Here, we present the first report on the identification and characterization of a lectin from S. apiospermum named SapL1. SapL1 was found using bioinformatics as a homolog to the conidial surface lectin FleA from Aspergillus fumigatus known to play a role in the adhesion to host glycoconjugates present in human lung epithelium. As expected from its homology with FleA, SapL1 recognizes fucosylated oligosaccharides independently of the fucose linkage. We finally demonstrated that SapL1 binds to bronchial epithelial cells in a fucose-dependent manner.

SapL1 was co-crystallized with α-methyl-fucoside and the structure of the complex was solved by molecular replacement at 2.3 Å resolution in the P21 space group using the coordinates of FleA (PDB code 4D4U34) as the search model. The asymmetric unit contained two monomers, assembled as a dimer with all 295 amino acids visible apart of the N-terminal methionine. SapL1 folds into the canonical six-bladed β-propeller with six-binding sites at the interface between blades typical for this family of lectin. Due to divergence in the tandem repeat sequence forming each blade of the propeller, the six binding sites of SapL1 monomer are not equivalent, but they share important conserved features. Hydrophobic interactions are observed between the C6 of the fucose and at least three residues of the protein (mainly isoleucine, tryptophan/tyrosine and leucine). The O2 and O3 hydroxyls make strong hydrogen bonds with a conserved triad of amino acids consisting of an arginine, a glutamic acid and a tryptophan. The O2 hydroxyl seemed to be the most versatile position, since it established interactions with an adjacent loop only present in four of the six binding sites (BPs 2, 4, 5 and 6). This is particularly interesting since the binding pockets that do not contain this loop (BPs 1 and 3) were mostly occupied by glycerol instead of fucose, indicating that those interactions could be responsible for enhancing the affinity and should be explored for development of inhibitors. The overall fold of SapL1 and FleA as well as the overall dimer are very similar with a rsmd of 1.2 and 1.26 Å, respectively. The affinity of SapL1 for L-fucose and α-methyl-fucoside was determined by Isothermal Titration Calorimetry (ITC) and the Kd was found to be 225 ± 1.52 µM and 190 ± 1.44 µM, respectively with stoichiometry fixed to 1 since the measurements were done in the presence of an excess of ligand.

>GHMSGVLQISFPAGIAAIRNNSSLRVYEAALDGGVREAQYEGRWAGGKPDNVIATGKIGTPIAATSVGFQYIRVYYVGADNKAREACWDGKGWYTGAFVKDVAPYSSIGAVFLGKNIVVRVYTQNHDNTIQEWVWDSPSTGWTAGANFGAALPGTAIAATSWGAGPYHIRVYFQDTNRNVIESGWDGSGWYTGGLKISNQSPRASLGATSWGESGSSLGIRLYYATQDNLIKEKAWDGGGGWYDGGFQQRSIPGSRVAAIPLPVLRVYLQNGTEVSGITEYAWNSGWVVGQAVLPPA[2x]> LGSMVATVKRTIRIKTQQHILPEVPPVENFPVRQWSIEIVLLDDEGKEIPATIFDKVIYHLHPTFANPNRTFTDPPFRIEEQGWGGF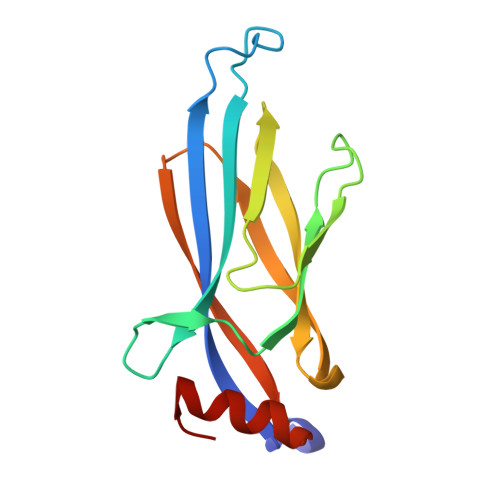PLDISVFLLEKAGERKIPHDLNFLQESYEVEHVIQIPLNKPLLTEELAKSGST> LPENVDWRKKGAVTPVRHQGSCGSCWAFSAVATVEGINKIRTGKLVELSEQELVDCERRSHGC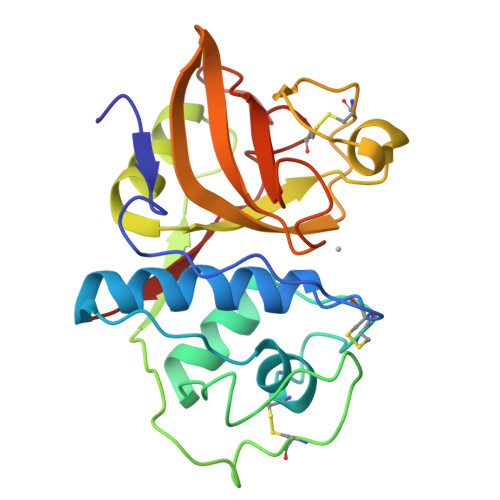KGGYPPYALEYVAKNGIHLRSKYPYKAKQGTCRAKQVGGPIVKTSGVGRVQPNNEGNLLNAIAKQPVSVVVESKGRPFQLYKGGIFEGPCGTKVDHAVTAVGYGKSGGKGYILIKNSWGTAWGEKGYIRIKRAPGNSPGVCGLYKSSYYPTKN> MFIKQSEKNTPKCLYKKKGKVRVLLTGSCKKLNTWKMHLWPVSPPQLLRIPPRNAELGEGTKIDDCNILQSMTLPQANVLIMLTPTRVLIYNFKPMALVASHERTMASLKEFGDNRSMKRSAPYNDIIEGLISKKDSQYLLWHQGKLIFYVMTDKNFLLTYQILKNCTNEIIFKEYGIPVIEPLLMSEEEANSAEYDYNNDDDTLTVFDKNSSSRIIQNGFGITKEKGFLHFLSNQENIDELPVKKLELRLKVVLKFDYEIIDMIGIKTFSKVGDGRYEEVLIVLFPHGLQILTISDFKVSKSSLVEVKKGSKTIVCNKQLMVLSHDSVEKQTIVSIIDIEKQAVEAIPLTDTPDELLTCLEVNGYLVVVYKEKIICFDTRIKKVSHSWKPPFVIKLCDKINDKILLLVSEDSVNIHFYTEFGNLLFATYFDEDDYNGDNNNDNSKDKNEKKAAEYKISDFVCLDKSLITVSHSGKYQVWKLWEEIKQTQFDFRNPKCYVLTNTNNDVIIYSPVTSSSINNDNLQVIKLPTKTFNNHIAFVKINSSLRLFATYVSNKNILLIHNLETNMWSSFADQNVLDLHWLGDNYLVCHMKNDDGSTNLKCLQIPLQEANPDVELSDYVMWEYNVPENTIVFSLHVNTLSRYKLLKMKSKNHNASEKQPDALLKTAEIILVTDTQTIVFDVISTVHPCGLNIIKKFYQYLKI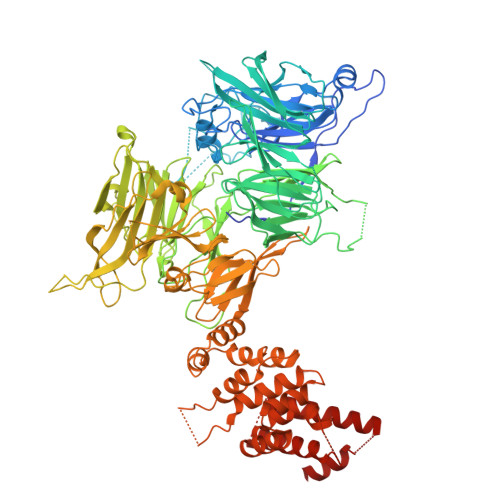NIPIDVLPNKIEWIINMKEGLLFFADRKFIKLGKVDGGGWQTLTLLDNIEKIIDVIRDEIFVVQGHNYVVYSLEDLWDDKKPLVSIPIEEDLYPISTTPETATTHTLHCIFNARFSKLVVKHQIYLDQLILAKLEDNTDLEDISHNYRFLKPYKFALEKILSTKILRSDSLDDILKLIKMYDNTDPEHNISPPTHSGMLEIISNCLRKIETKYWNHLFTNLKMTPRDLLALCIEENEAKMLGVLLLVFLNYDEKDLGDDLHFKKSDLGTEESKALNDNSTKKSEKSVTNLLKXXXXXXXXXXXXXXXXXXATDXXXXXXXXXXXXXXXXXXXXXDRENNTQXXXXXXXXXX>APEGYRKLLDVQIFKDSPVVGWSGSGMGELETIGDTLPVDTTVTYNGLPTLRLNVQTTVQSGWWISLLTLRGWNTHDLSQYVENGYLEFDIKGKEGGEDFVIGFRDKVYERVYGLEIDVTTVISNYVTVTTDWQHVKIPLRDLMKINNGFDPSSVTCLVFSKRYADPFTVWFSDIKITSEDNEKSAPAIKVNQLGFIPE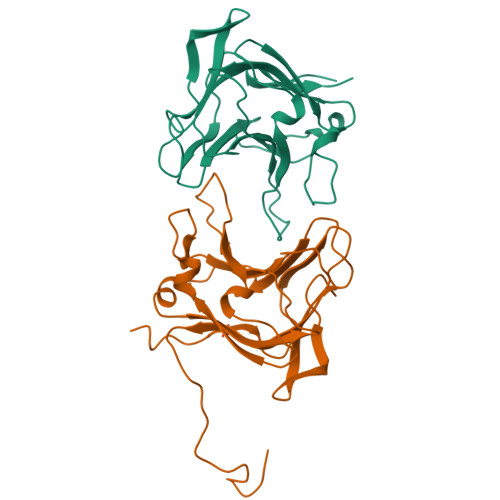AEKYAL[2x]>MSMAMSQSNRELVVDFLSYKL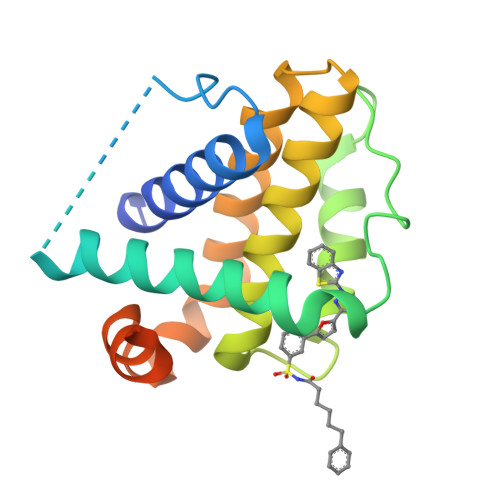SQKGYSWSQFSDVEENRTEAPEGIPMAAVKQALREAGDEFELRYRRAFSDLTSQLHITPGTAYQSFEQVVNELFRDGVNWGRIVAFFSFGGALCVESVDKEMQVLVSRIAAWMATYLNDHLEPWIQENGGWDTFVELYGNNAAAESRKGQERLEHHHHHH[2x]>MAHHHHHHMTTNTQITEDRILILDFGSQYSQLIARRVREAGVYSEMYAFDMSEEDIRAFKPNGIILSGGPESVHE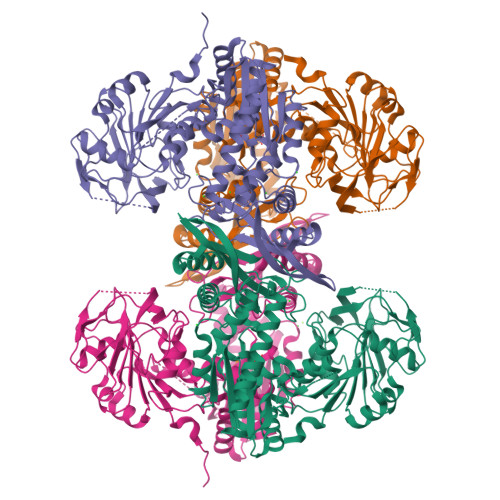EGSPRAPQVVFELGVPVLGICYGLQTMSEQLGGKVEPGTVHEFGYAEVDIVKRDQLIGNLQDRENQLHVWMSHGDKVSQIPEGFTITASTPSCPVAAVSDETRRFYGVQFHPEVTHTAKGEELLSNFVHKICGCGGLWTPEHIIDLRVEQLREQIGNEKVLLGLSGGVDSSVVAALLHKAIGDQLTCVFVDNGLLRLNEGDQVMQMFAENMGIRVIRADAEARFLNALAGVTDPEAKRKIIGREFIEVFAEEARKLDGVKFLAQGTIYPDVIESAASKQGKAHVIKSHHNVGGLPDDLAFELVEPLRDLFKDEVRKLGTTLGLPHSMIYRHPFPGPGLGVRILGEVKKEYADILRLADDIFMQELRDSGWYDKTAQAFAVFQPVKSVGVVGDGRRYAWVIALRAVETVDFMTARFAHLPYELVDKISTRIMNEIKDVSRVVYDVSSKPPATIEWE[4x]N-(1-{[(3-tert-butylbenzoyl)amino]methyl}cyclopentyl)-2,1-benzoxazole-4-carboxamide | C25 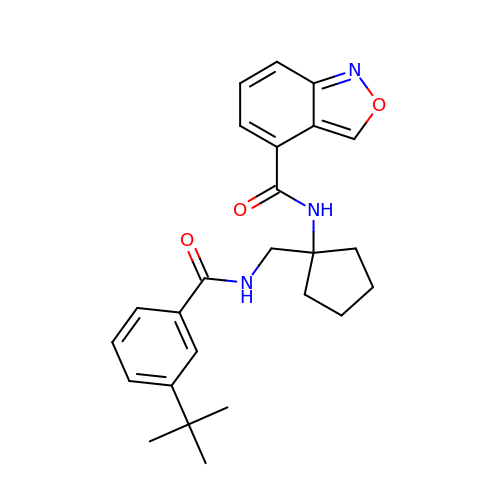H29 N3 O3 | ZVPHHRCZSPAOCC-UHFFFAOYSA-N>MKQKPAFIPYAGAQFEPEEMLSKSAEYYQFMDHRRTVREFSNRAIPLEVIENIVMTASTAPSGAHKQPWTFVVVSDPQIK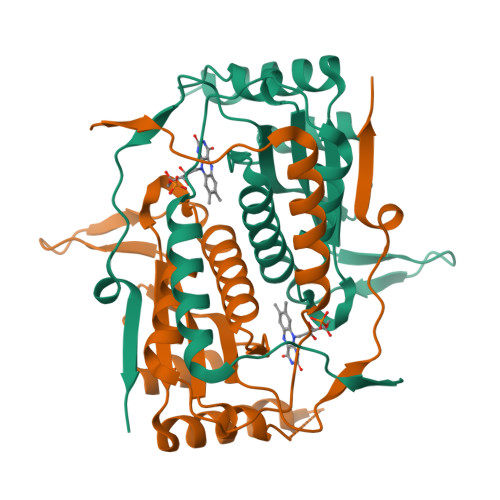AKIRQAAEKEEFESYNGRMSNEWLEDLQPFGTDWHKPFLEIAPYLIVVFRKAYDVLPDGTQRKNYYVQESVGIACGFLLAAIHQAGLVALTHTPSPMNFLQKILQRPENERPFLLVPVGYPAEGAMVPDLQRKDKAAVMVVYHHHHHH[2x]> NLYQFKNMIECTVPARSWWDFADYGCY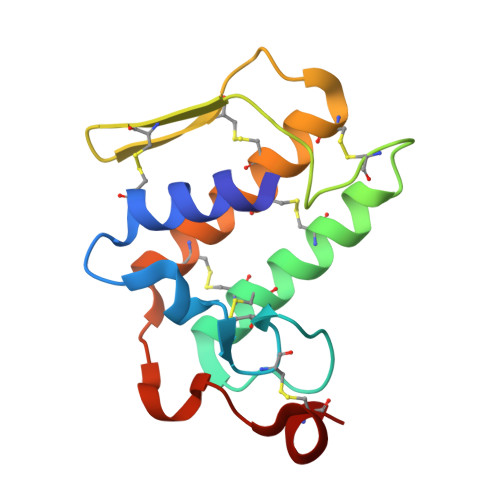CGGGGSGTPTDDLDRCCQVHDNCYNQAQEITGCRPKWKTYTYQCTQGTLTCKGRNNSCAATTCDCDRLAAICFAGAPYNDTNYNIDLKARCQ> MADVLTELPGVGPSTADKLIEGGYLDFMKIATATIGELTDIEGISEKAAAKMIMAARDLCDLGFKSGVELLKQRQ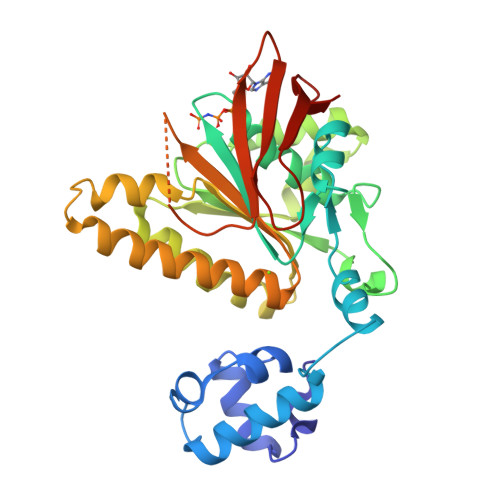SVWRLSTGSTELDTVLAGGIESQSVTEFAGMFGSGKTQIMHQTCVNLQMREKIFADLEGVVEEELEAPKAVYIDTEGTFRPERVVQMAEGAGIDGQTVLDNTFVARAYNSDMQMLFAEKIEDLIKGGNNIKLVIIDSLTSTFRNEFTGRGKLAERQQKLGRHMATLNKLADLYNCIVLVTNQVAAKPDAYFGVAEQAIGGHVVGHAATFRFFLRKSKGDKRVAKLYDSPHLPDSEAVFRITEKGIQD>LVPRGSHMTNDTSGVLTIATTHTQARYSLPEVIKAFRELFPEVRLELIQGTPQEIATLLQNGEADIGIASERLSNDPQLVAFPWFRWHHSLLVPHDHPLTQISPLTLESIAKWPLITYRQGITGRSRIDDAFARKGLLADIV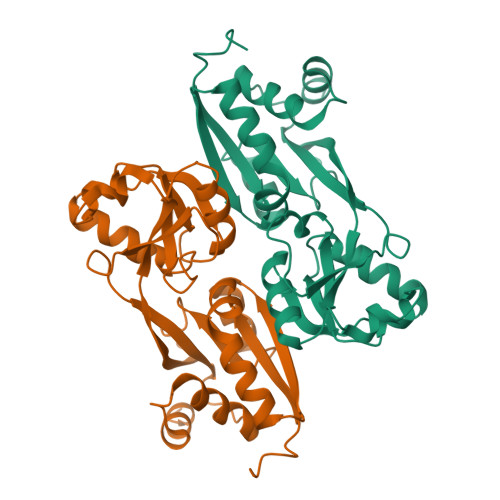LSAQDSDVIKTYVALGLGIGLVAEQSSGEQEEENLIRLDTRHLFDANTVWLGLKRGQLQRNYVWRFLELCNAGLSVEDIKRQVMES[4x]>[2x]MKIVVMGDSDTVVGFRLAGVHEAYEYDESLESVERARNKLRELLER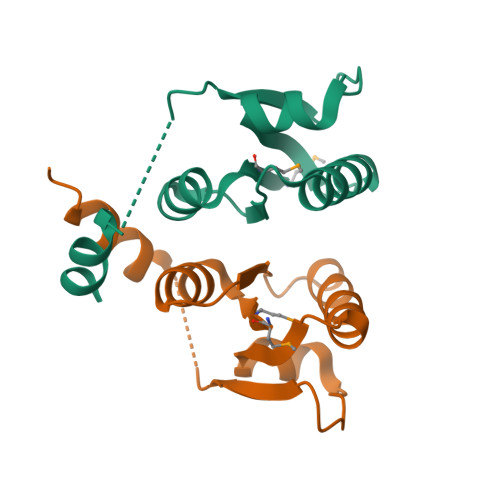DDVGIILITERLAQRIGSLPEVKFPIILQIPDKFGSIYGEDILRDVVRRAIGVELKRLEHHHHHH>[2x]MTHYELQALRKLLMLEVSEAAREIGDVSPRSWQYWESGRSPVPDDVANQIRNLTDMRYQLLELRTEQIEKAGKPIQLNFYRTLDDYEAVTGKRDVVSWRLTQAVAATLFAEG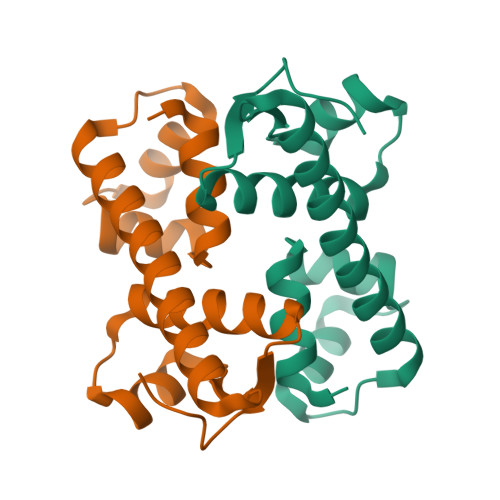DVTLVEQGGLTLE> GMNSPKNSLYEEKSGHYYNAVNPNLLKHIKKEWKEVLDIGCSSGALGAAIKENGTRVSGIEAFPEAAEQAKEKLDHVVLGDIETMDMPYEEEQFDCVIFGDVLEHLFDPWAVIEKVKPYIKQN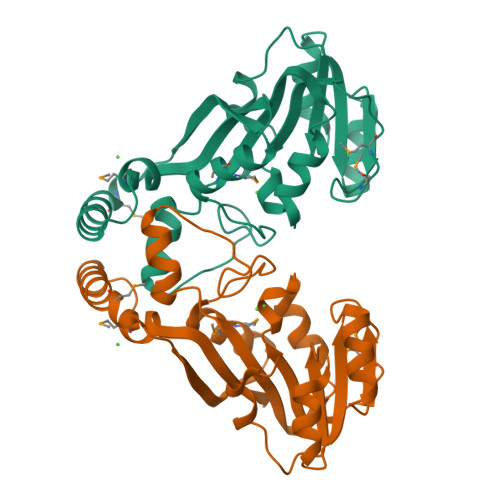GVILASIPNVSHISVLAPLLAGNWTYTEYGLLDKTHIRFFTFNEMLRMFLKAGYSISKVDRVYVDHKMYEPLIEELYGICKKYRLGSGFMAETVVFQYIIEAEKSQL>MRLEIPNHTERFGVVRLHEVQRILELDSGRVRDESPAVGLRRLDDADLRDVLEQTAIVVPTRNERLKLLEGVLSGIPHEALILVASNSSPDRFQMERDLLEEFAHLTERPALIFHQKDPALAEALRAGGYPHPIGEDGLVRSGKAEGMILALVFAALSGRRYVGFIDADNYFPGAVWEYVRAYAAGFLMAKTPFAMVRILWRYKPKLTEDEGVVFRRYGRVSERNNRALNQLIGGVSGFETDVVKTANAGEHAMSLGLALRLPLASGYAVEPQELVSLLELYGGVFPLEDEEVLQHGVEIFQIETRN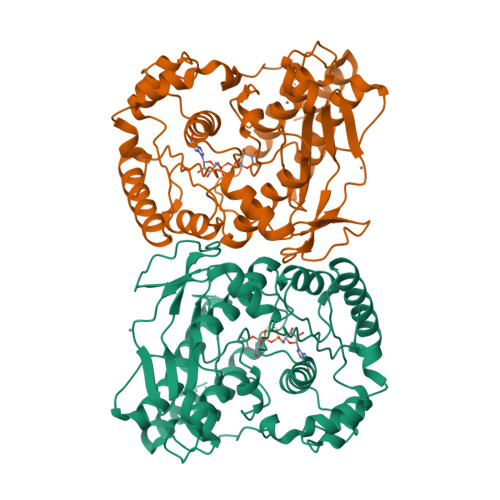PALHENKGDEHIRDMLLACLATVYHSKLATEEVRQSVLEELQAAGALAPGEEPPPPVLYPPLSSLDLQAVRKALRGHFSRFRVP[2x]4-cyano-N-cyclopropyl-N-[(thiophen-2-yl)methyl]benzamide | C16 H14 N2 O S 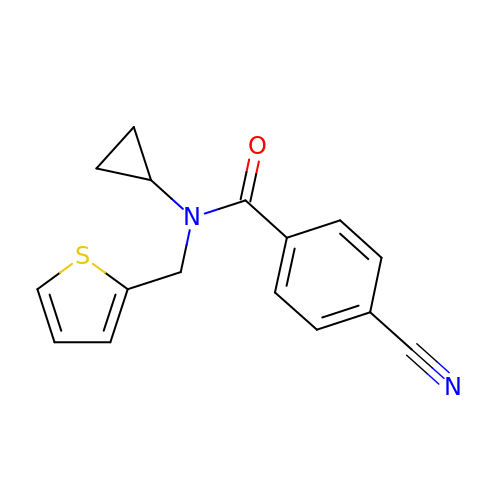| WYAGGMZTARRIDX-UHFFFAOYSA-N(3R,4S)-N-{2-chloro-5-[(cyclopropylamino)methyl]benzyl}-N-cyclopropyl-4-{6-[2-(2,6-dichloro-4-methylphenoxy)ethoxy]pyridin-3-yl}piperidine-3-carboxamide | C34 H39 Cl3 N4 O3 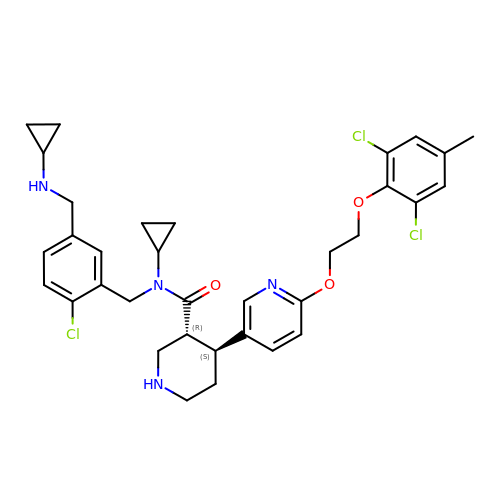| MUNGQQYSICIEKG-IZLXSDGUSA-N>MSLIYAQILAGGKGTRMGNVSMPKQFLPLNGKPIIVHTVEKFILNTRFDKILISSPKEWMNHAEDNIKKYISDDRIVVIEGGEDRNETIMNGIRFVEKTYGLTDDDIIVTHDAVRPFLTHRIIEENIDAALETGAVDTVIEALDTIVESSNHEVITDIPVRDHMYQGQTPQSFNMKKVFNHYQNLTPEKKQILTDACKICLLAGDDVKLVKGEI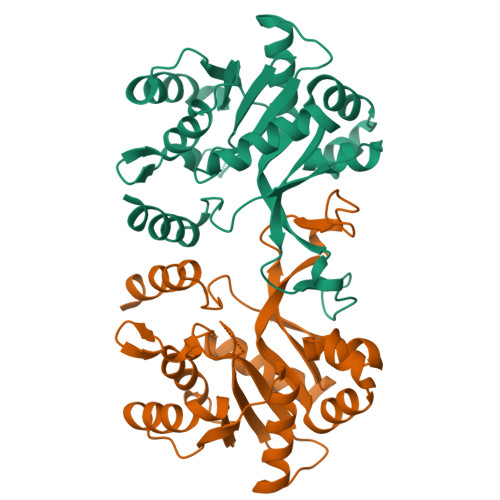FNIKITTPYDLKVANAIIQERIANEGHHHHHH[2x]>MVPISPIETVPVKLKPGMDGPKVKQWPLTEEKIKALVEICTEMEKEGKISKIGPENPYNTPVFAIKKKDSTKWRKLVDFRELNKRTQDFWEVQLGIPHPAGLKKKKSVTVLDVGDAYFSVPLDEDFRKYTAFTIPSINNETPGIRYQYNVLPQGWKGSPAIFQSSMTKILEPFKKQNPDIVIYQYMDDLYVGSDLEIGQHRTKIEELRQHLLRWGLTTPDKKHQKEPPFLWMGYELHPDKWTVQPIVLPEKDSWTVNDICKLVGKLNWASQIYPGIKVRQLSKLLRGTKALTEVIPLTEEAELELAENREILKEPVHGVYYDPSKDLIAEIQKQGQGQWTYQIYQEPFKNLKTGKYARMRGAHTNDVKQLTEAVQKITTESIVIWGKTPKFKLPIQKETWETWWTEYWQATWIPEWEFVNTPPLVKLWYQLEKEPIVGAETFYVDGAANRETKLGKAGYVTNKGRQKVVPLTNTTNQKTELQAIYLALQDSGLEVNIVTNSQYALGIIQAQPDKSESELVNQIIEQLIKKEKVYLAWVPAHKGIGGNEQVDKLVSA[2x];>MAHHHHHHALEVLFQGPISPIETVPVKLKPGMDGPKVKQWPLTEEKIKALVEICTEMEKEGKISKIGPENPYNTPVFAIKKKDSTKWRKLVDFRELNKRTQDFWEVQLGIPHPAGLKKKKSVTVLDVGDAYFSVPLDEDFRKYTAFTIPSINNETPGIRYQYNVLPQGWKGSPAIFQSSMTKILEPFKKQNPDIVIYQYMDDLYVGSDLEIGQHRTKIEELRQHLLRWGLTTPDKKHQKEPP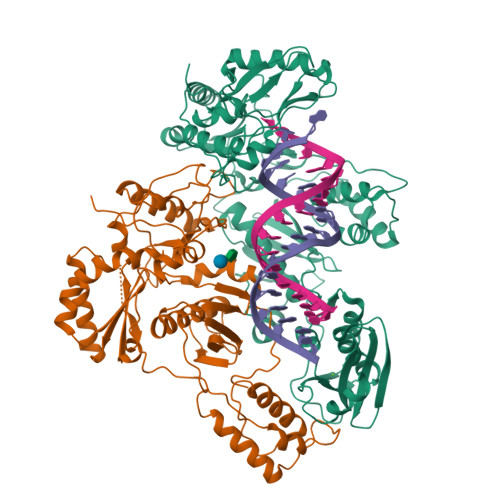FLWMGYELHPDKWTVQPIVLPEKDSWTVNDIQKLVGKLNWASQIYPGIKVRQLSKLLRGTKALTEVIPLTEEAELELAENREILKEPVHGVYYDPSKDLIAEIQKQGQGQWTYQIYQEPFKNLKTGKYARMRGAHTNDVKQLTEAVQKITTESIVIWGKTPKFKLPIQKETWETWWTEYWQATWIPEWEFVNTPPLVKLWYQ[2x]>[2x]NSIIGEKYRWPHTIPYVLEDSLEMNAKGVILNAFERYRLKTCIDFKPWAGETNYISVFKGSGCWSSVGNRRVGKQELSIGANCDRIATVQHEFLHALGFWHEQSRSDRDDYVRIMWDRILSGREHNFNTYSDDISDSLNVPYDYTSVMHYSKT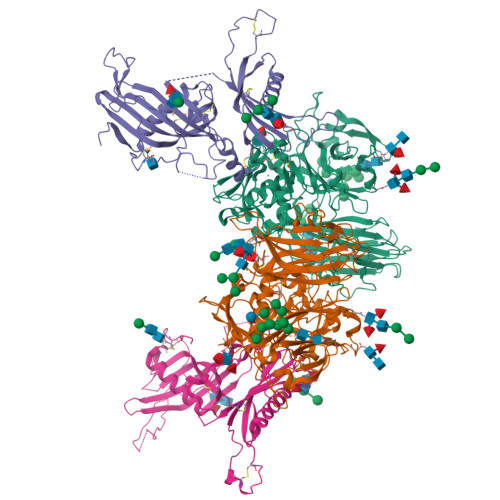AFQNGTEPTIVTRISDFEDVIGQRMDFSDSDLLKLNQLYNCSSSLSFMDSCSFELENVCGMIQSSGDNADWQRVSQVPRGPESDHSNMGQCQGSGFFMHFDSSSVNVGATAVLESRTLYPKRGFQCLQFYLYNSGSESDQLNIYIREYSADNVDGNLTLVEEIKEIPTGSWQLYHVTLKVTKKFRVVFEGRKGSGASLGGLSIDDINLSETRCPHHIWHIRNFTQFIGSPNGTLYSPPFYSSKGYAFQIYLNLAHVTNAGIYFHLISGANDDQLQWPCPWQQATMTLLDQNPDIRQRMSNQRSITTDPFMTTDNGNYFWDRPSKVGTVALFSNGTQFRRGGGYGTSAFITHERLKSRDFIKGDDVYILLTVEDISHLNSTQIQLTPAPSVQDLCPSK;>[2x]MGLLRLLVLCTLAACCMARSPPAPPLPQRPLSPLHPLGCNDSEVLAVAGFALQNINRDQKDGYMLSLNRVHDVREHYQEDMGSLFYLTLDVLETDCHVLSRKAQKDCKPRMFYESVYGQCKAMFHINKPRRVLYLPAYNCTLRPVSKRKTHTTCPDCPSPIDLSNPSALEAATESLAKFNSKSPSKKYELVKVTKAMNQWVSGPAYYVEYLIKEAPCTKSQASCSLQHSDSEPVGICQGSTVQSSLRHVPLIQPVEKSVTVTCEFFESQAQVPGDENPAVTQGPQKLPQKNTAPTSSPSVTAPRGSIQHLPELDDEKPEESKGGSPEEAFPVQLDLTTNPQGDTLDVSFLYLEPGDKKLVVLPFPGKEQRSAECPGPEKENNPLVLPPHHHHHH>[12x]MRVIFSEDHKLRNAKTELYGGELVPPFEAPFRAEWILAAVKEAGFDDVVAPARHGLETVLKVHDAGYLNFLETAWDRWKAAGYKGEAIATSFPVRRTSPRIPTDIEGQIGYYCNAAETAISPGTWEAALSSMASAIDGADLIAAGHKAAFS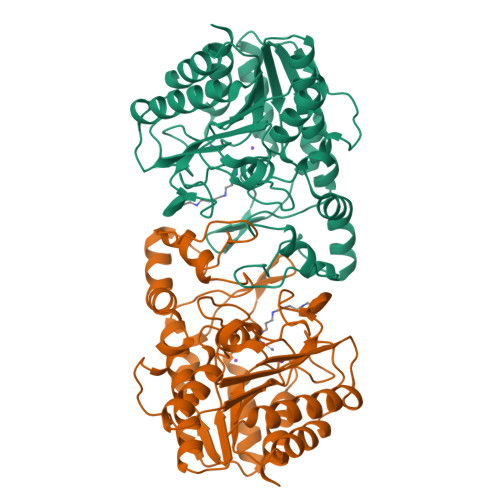LCRPPGHAAGIDMFGGYCFINNAAVAAQRLLDKGAKKIAILDVDFHHGNGTQDIFYERGDVFFASLHGDPAEAFPHFLGYAEETGKGAGAGTTANYPMGRGTPYSVWGEALTDSLKRIAAFGAEAIVVSLGVDTFEQDPISFFKLTSPDYITMGRTIAASGVPLLVVMEGGYGVPEIGLNVANVLKGVAG(2~{S},3~{S},4~{R},5~{R})-5-(6-aminopurin-9-yl)-3,4-bis(oxidanyl)oxolane-2-carboxamide | C10 H12 N6 O4 | 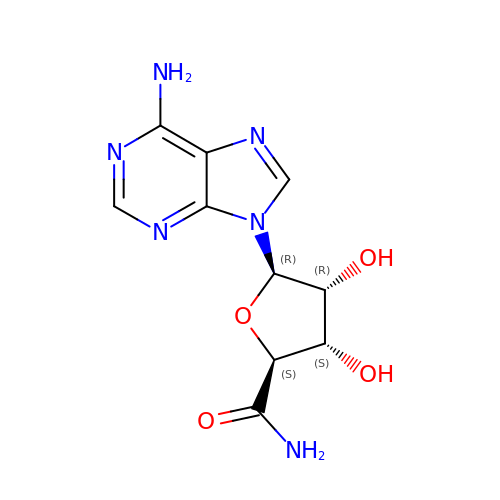BLMHAOGGJQDPLX-LKCKTBJASA-N>[12x]SPNIKIFSGSSHQDLSQKIADRLGLELGKVVTKKFSNQETCVEIGESVRGEDVYIVQSGCGEINDNLMELLIMINACKIASASRVTAVIPCFPYARQDKKDKSRA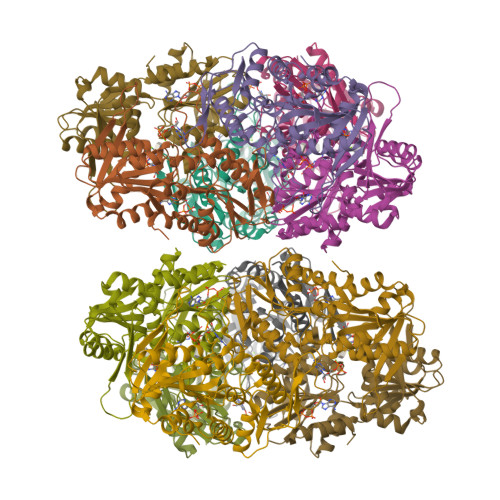PISAKLVANMLSVAGADHIITMDLHASQIQGFFDIPVDNLYAEPAVLKWIRENISEWRNCTIVSPDAGGAKRVTSIADRLNVDFALIHKERKKANEVDRMVLVGDVKDRVAILVDDMADTCGTICHAADKLLSAGATRVYAILTHGIFSGPAISRINNACFEAVVVTNTIPQEDKMKHCSKIQVIDISMILAEAIRRTHNGESVSYLFSHVPL> NE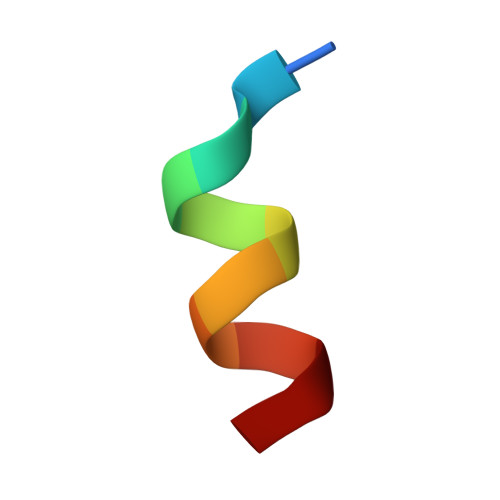ALLRYLLDK> APSYPEYTREEVG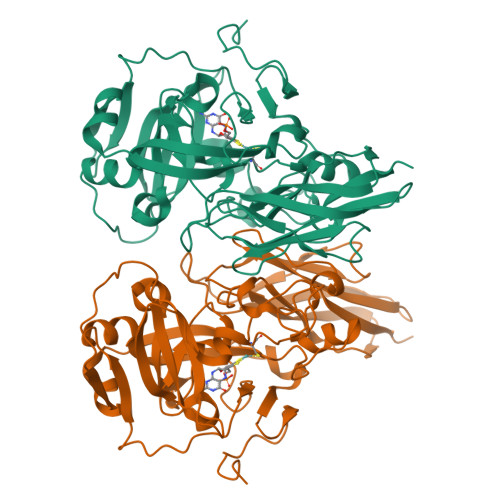RHRSPEERVWVTHGTDVFDVTDFVELHPGGPDKILLAAGGALEPFWALYAVHGEPHVLELLQQYKVGELSPDEAPAAPDAQDPFAGDPPRHPGLRVNSQKPFNAEPPAELLAERFLTPNELFFTRNHLPVPAVEPSSYRLRVDGPGGGTLSLSLAELRSRFPKHEVTATLQCAGNRRSEMSRVRPVKGLPWDIGAISTARWGGARLRDVLLHAGFPEELQGEWHVCFEGLDADPGGAPYGASIPYGRALSPAADVLLAYEMNGTELPRDHGFPVRVVVPGVVGARSVKWLRRVAVSPDESPSHWQQNDFKGFSPCVDWDTVDYRTAPAIQELPVQSAVTQPRPGAAVPPGELTVKGYAWSGGGREVVRVDVSLDGGRTWKVARLMGDKAPPGRAWAWALWELTVPVEAGTELEIVCKAVDSSYNVQPDSVAPIWNLRGVLSTAWHRVRVSVQD> MAYPYDVPDYAAAVKKLTDKQKSRLWELQRNRNFQASRRLEGVEMPLV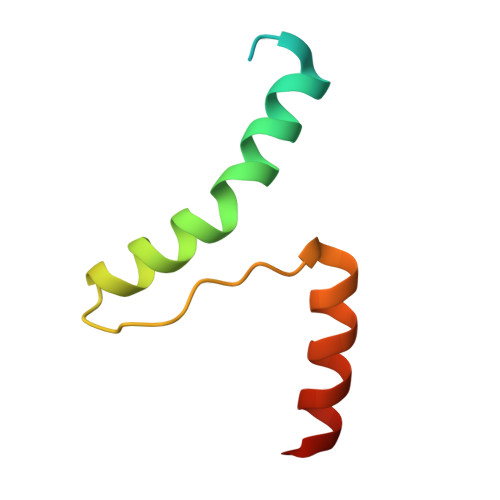TLTAAEALARLEELRSHYER>XGQLEQELAALDQQIAALKQRRAALKW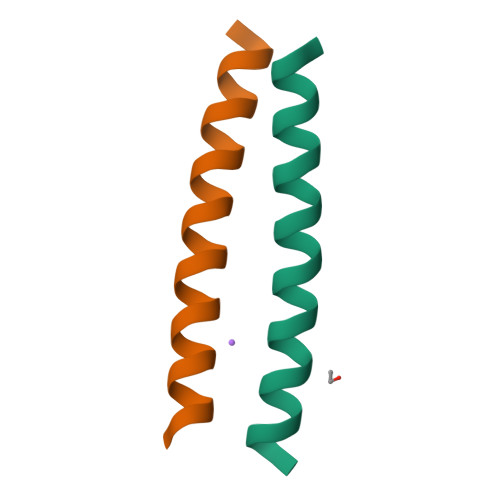QIQGX[2x]> GMLSNLESSIQSPKSGEYQCLAALNLYDSPECTSLATQAAVGRHLQVTSNQQGAAVEVCLCEDDYPGWLSLGDL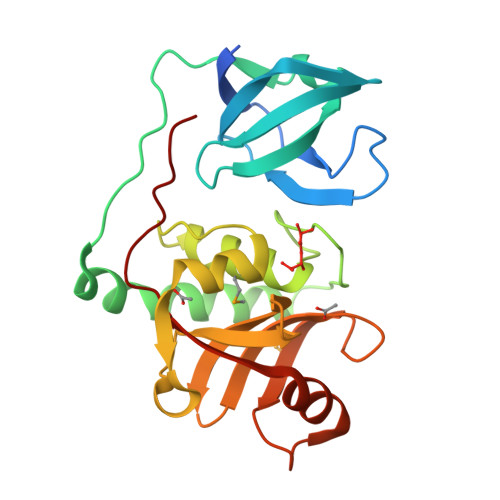GLLKPATVLYQAKSFSESEIKKLLPGAIAFTQKAMQQSNYYLWGGTVGPNYDCSGLMQAAFVSVGIWLPRDAYQQEAFTQAITIDELAPGDLVFFGTPVKATHVGLYLGDGCYIHSSGKAQGRDGIGIDILSEQGDVVSRSYYQQLRGAGRVVKSYKPQRH> MVSNASALGRNGVHDFILVRATAIVLTLYIIYMVGFFATSGELTYEVWI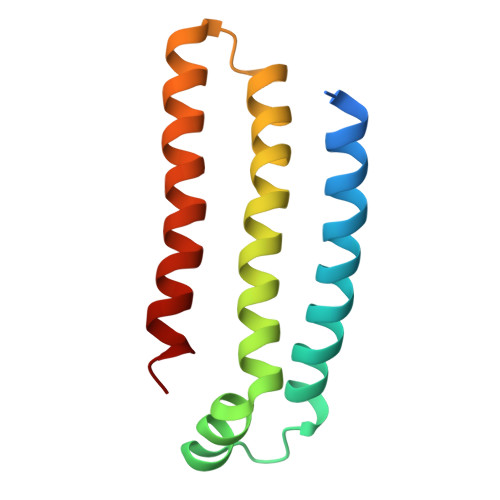GFFASAFTKVFTLLALFSILIHAWIGMWQVLTDYVKPLALRLMLQLVIVVALVVYVIYGFVVVWGV D-GLUTAMINE | C5 H10 N2 O3 | 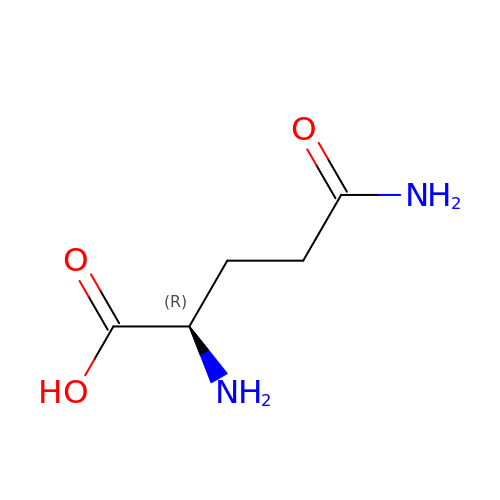ZDXPYRJPNDTMRX-GSVOUGTGSA-N>MSASAQQLAEELQIFGLDCEEALIEKLVELCVQYGQNEEGMVGELIAFCTSTHKVGLTSEILNSFEHEFLSKRLSKAR[11x];>[12x]KQVSWKLVTEYAMETKCDDVLLLLGMYLEFQYSFEMCLKCIKKEQPSHYKYHEKHYANAAIFADSKNQKTICQQAVDTVLAKKRVDSLQLTREQMLTNRFNDLLDRMDIMFGSTGSADIEEWMAGVAWLHCLLPKMDSVVYDFL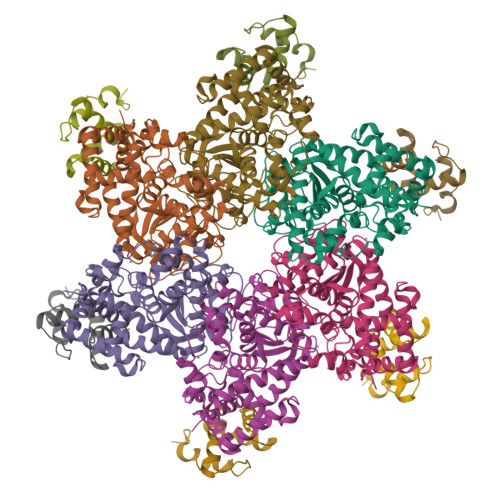KCMVYNIPKKRYWLFKGPIDSGKTTLAAALLELCGGKALNVNLPLDRLNFELGVAIDQFLVVFEDVKGTGGESRDLPSGQGINNLDNLRDYLDGSVKVNLEKKHLNKRTQIFPPGIVTMNEYSVPKTLQARFVKQIDFRPKDYLKHCLERSEFLLEKRIIQSGIALLLMLIWYRPVAEFAQSIQSRIVEWKERLDKEFSLSVYQKMKFNVAMGIGVLD> GIDPFTKHGQKECDNALRQ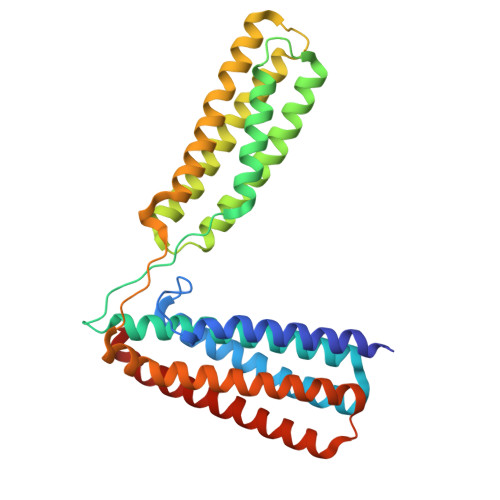LETVRELLENPVQPINDMSYFGCLDSVMENSKVLGEAMTGISQNAKNGNLPEFGDAIATASKALCGFTEAAAQAAYLVGVSDPNSQAGQQGLVEPTQFARANQAIQMACQSLGEPGCTQAQVLSAATIVAKHTSALCNSCRLASARTANPTAKRQFVQSAKEVANSTANLVKTIKALDGDFTEENRAQCRAATAPLLEAVDNLSAFASNPEFSSVPAQISPEGRAAMEPIVISAKTMLESAGGLIQTARALAVNPRDPPRWSVLAGHSRTVSDSIKKLITSMRDKAPGQL> MLKCSLCYLASKVTAGNAKNQAGHPRRKAKLFHVVPGTPVTPFEKLKEQRRRFGQDRHSRLPEYRPGNNVRMDPNTYTLYATKKGVMTIRESRINPKYKWLDVEPDIQKVYRSRELRRALQEREMASMAVGENSNYRVELDLLLEPDWRERVMHVPKATERFKDPNLFTRGVVNELSPLDRYSYT;> MLRNTDVRLFSTFALNPETSVAPHGPPRGLVNRYVSMGLPPWAAWCNKVNRYSLYRMSGVTQRSFLPKPPQEMDVIWLNERVRERVRTSRQVQNVYRQLKYPYVKTGIHYSDVLDHWVQVPMVEAAMFEVEKDGGFDNFILKRSGPELRSTYGERIRRHILVRQKEIQKNFVLQKQAQMLVESMEKEILPMEDGKKVEEVLEKYGIDKEQLLRDIARAAVAKKQQLASAVPQPSHVEVSTN;> MQRNLTKLSAAAFYEFVDNNFLNNKRPPVPGGSWTVEVLRNKSLADLQHIWFLLLKERNMLKSMKEHYLRHQEELGAMPAPSRLKMIDESMRNIKRVVKERDEEATARAVEIFKERLKRGIYRYPPGPPPPPGAHDKTSVVKVELSCYVEEERLRELFGRYDVFEPHKGIVRVELKLPDEVLKQKEEAEQLWTQYMAECSDVKAYHQWSTAAPSAYDYTEVELAPGIFANDAISDKGGKHSGDTETHEGVIVAARVPVPPPKEKQPPPKNPLERLKAERRSYLARTTIQLGYFPNVTLPPPRYETVEAVPRPVHPDEIEGPWEAYITYDREDGLSYAQSLGITTIGVATVLGLTEHVREPQPYAVVDPVYCEALRRERAREETLMKWPHVPEWKYEYSTYTRKHLADIVQYNYTNVVDYVDREVLLTGKSVWECPIHIDHTCGGSKTVPPHAKKPVRYMDAGIANVGVTDI;> MMRRMWVPTFSAQQQHLHHAMVLKMSTYASTPSGNGVTSAASNEEMNLHDAAAIAPGPYRRVGNIFIVHCDDHPFKHSWEVNRMLRELRLEFKGQTTIVPDIPQVRKRIWRVRHIVKVDVLDLDEAKALIGVPEHISFTDLASQLPPSFGRVKAVPSPVIRSKMNFMKLRRMRLRDVLHRDALELRLLELKRSAMKNAEQQKHAQKDERTDNKEGEKC;> MVLHKWAVVSRSAPPPRGLRPIARTIPTHPRLRPVDYKIPYVLRTFIKDRHTSEVQHLENRGMFAEELSIERSRFPRFHSTFTIQTDGSLNEREFEFAVPPIVTLFHDRLSAHRERQLELAKIGKLRKERNWETEQKGEESVSMACNALAFPYCIPKNMLKRSRVVDPLNSKSSTQGVTSGGG;> MFRRTFFTPMIAQPTLLMLGNKGGTPKRKKNPMQLRRKVYGLHFKEKYLKMEEWYYCPLCAEPKKPGEWCRREDCRQIKP;> MLSSTALLLRGQYKTRLKKRMVGFIPKVIPRKIKNNMVALRSEANTGHMEGYLKTETERLDATGRKVQKVLWDPVLQRHCLFKETKIKGPFMTKSAIAKKVDFPIGGAEKMLKK;> MGSEESNNICAYKRTISLAKIYIVLLVKTAMLRYSRLCFPKMGCEEITRKARRVQLQPTEYLAQHRMQVWQLRFKEMGPPFSRVWVALGGKMRRRRVGRQVDVKDMRYYWRPIEPQYQRLYMSRLRIRDHSNKLRQPMRLRATNADIGSGSSSIEWERASNRKYGAMLAPPKRQDFEFRVV;> MRGTTKPMLFLCSTAVRLNFFPLGLSAGPLNSHILLPRNNFDGRTTHGMKKIQGQSKDPQMVMSRDELKLRCEYCRFEWIHDTLCVRCPAQPSHDQREMWLHSTWMWGKQQPYKYYKYMPAVRNPRTGMPMAREDARSMNNERRGQGLTTRTLNLEKERRGISRDVSRIGQYNTRWKTRFPFPT;> AAAAAAAAAAAAAAAAAAAAAAAAAAAAAAAAAAAAAAAAAAAAAAAAAAAAAAAA;>AAAAAAAAAAAAAAAAAAAAAAAAAAAA[2x];> MRSLIAMRRRFVSGTWTIAVSTQQRHRSGSGPGDKRIRTDWYRCYPSLMREKDRDMYHCYYPYLFDHGDKMSLYPKIPENPREWQPEQLQTTYDAIREDKYDAFIRLREKFPELYQDTRAWDNPPPFGEFNMFYSVRFGMVGVKAFTCKDYDELGNQFDCTAFWFPDNQVVKHSTRNGEVGTDKVYVGAMNVPVEFHKPHVAAFYKAAGVPVKHVCAGFPITPDAYAPVGTKLDVRHFKPGQEVTITFQNTDYGFRGVMFRHGFDGGYVWLGDSRWQRRPGAMGTEGQKRIYPGHRMAGQTGAAAETYQGVPVWRIDYKNSLIYLPTLLDADVGTYVRFSDTINTKGLTLWNEHRGLPAFPTFIPPEDEDLSKLATDECQLKSPPLYMYFRDEFPATQLVSQADVEDAKSAKPATAPPKKKVYDMKKYYEARKKYRQSMQKARKYKLMGLRTKAHEKQEEARRAKILKYKRMK;> MRRVSFSVVLATFGKRHSSIFSPRYDWRTSGVHDIAPRDEGDFLYQGPQHVLPGAHPLPLHHPHNTITRPVISPYIPSPQRSHPYFTAPLPELPHFSTTKPIVYTYGTMKERIIAPVFNLKNEVIYTRELDPFIFGMYPEVEELSKNLTYWMVRCQNFASKWDYETREIWRKAKKNWPNTGMGMPRVGNRKNHLYTWGGRTKPSKPWNMLMPTMDVKTWSKSNRMMLTLKMLQGRLQVVDRLTLEEPTQECYLELCRNMSWDVRHTGGGVLFMDGGSRITPSSEFDRAFFFGSFFNGRNKIVRPTVLCDEQYDYNKTAAKQRMKGPKGAKNPIPINRFNAYDAMKHDRLVITEGALMQLEDELYEHKLQILPPHIRNQLPEYGYLDSEALGDCVPSLKTIQMEAAARTEEAESDMYKSFIDNPYNPWKDNMDASYAVDGADGTVQKFVDGKKVSWSMLS;> AAAAAAAAAAAAAAAAAAAAAAAAAAA;> MRRTVVQRVAPWVPPPRHDIKVTMPPPPGGEVGGRFGVSQGYSDRLARTPYWKRMALSTYKLRMMENATRYPMSEHRPGEYDIRYLPTPYPCTIRNRPLLEVGEPRQIPSIRIPVIFLVNLFDEAKGCWFGRRYETVYVERQFMREELMPQRYAIYATPEAYKLLGLPVVNHHTHEEIPKTPREYEKLLERQRYDEERWKYTIEYLFRKYEDGPPELLDRPEDGWDGSEEIALSSVAGAGRDGVVSQRKGPVKQRKARKIKLF;> MSPASPLPVAALSRLRITHRSFLTRSRGRHVCRSAVGVEYRPEQQKKVLDHSYARVINAEVVHGDEQKFWGERRTFYTQRNIFFPMWDRCAQALILITREVPRVPQEMAFRLMAVFLKLMLLPRLMMNTELMLPMWIASNAEGAMAAAKDGSKGKEQSSKQQGESKDDAKKEGDNTK;> MLRACGVLQLRARPKTVCVEPGSNRLPEALVVEKARDIFGRPEFPGKRVLHNWRFFIKAGKAATGPPVGQEFSKLGLKAMDFAKVFNDRTKPHFKEDVELIVRIQVYFDKSYLFTIEPPPTAWFILRALRKKRRETGPVPLRGHYCALMTLEMAYEIAKMKPLCWGRPEYPLLETRVRRVVGQARRMGVCFIGVDTPYSSPVKDMTEQQYTEECERYRRIHMEQYTTLRQRELEEAPLIERLHRPNMSPLTDEQIEEGLRDPCLLDTLWRASHPLSPYHRDLRERELARRYLNARGWVKDMTPEEMRIVFMNYRLPEGEKRKQMDEAAMSGEVYWTRDGAQL;> MQRSTRIVMAPFKSVLRRHKHHPEGLPLYNDMSKQWLCREGERWWLLDARGEQLPRVAAVAAQYITGQHRPDFTPGMITGDHVVIVNIKDVVMVGDQWIRVPITWQTAYPGGKYRIRLTDMYERDPCMLMWWFLKDEVNRHFVRKLKTRIAPLEKAWLYEDSIHPHADKNPRPLCWTDPEVKGWKYRDPQFIRRWKPNEFMH;> MLSVSPPLRRYRLFHPRREAIPMHMCPAKTIFPLINSNNLLVKTRNSWEDFTGRKEFDEDHPLPVVGSRLNGRTTQHKWNHWDQYLNPQITQSIKDLTPTPEYVGMRCGHNMIKMGWMKIGGSWKYSRGYNDRRRVFARGQWQERKMTPRFMLAPRVSAGGPRNRYEGKLVFSPLRLSKLLWAIDTGRINPNEVITLYHLRQANVVGEREIVWPGFVLISNGVRRVPYPIHIELQNASAESIRLIEEAGGSFTCVYMTHEGLYQELHPEEYPIFMDQELPERRGLESLATNPSKRGWLTRWYEDSSKYAHPAAGRRYSHYLKPPTERDFPATVEEYEMVKHHQKWHLNQPGTGTLLPWHSYNTADLVKRAAGRL;> MPSPFQQTLLARAYHYVHPKTGRPIRQFRRYGDPRYINNEAALIRGQWGLITADFGMVTQSQMENARLAILRRLPRGSFTLTMHTDYEEFPVVKKSPESRMGAGKANIHHFAFKFTTGVPLFEIMPISARRLNQAEAEGIFLAGRPFIPLQTVVVPQGRVDEYHVFK;> MLRITLLVVGRAPPVIGCTRKARYAGIDDNPTITYKPWDTTEPLMADYGWTRGKLPKFRARSPFHRQQIARRMVTEMIRKDYCIVGGARAPALRILADHVVELAKAGDTDSRQQLAYFLHDPLMVDKAFDEYPRRFKDMNAKYAMMTRLKSRRRTDAVAMYFVEYKNRDMSDNHKGEDYSAGPERFFLPPRIVETEKGIQRPPHMQMAFDRWASKFKTEEFHHWWRLRHAKLRYWGVRNVPHPSDVDPLWTEKEEEEWHNEMLANTGEYEDLDLDDESYTAAGEGGEPSPAGDGPQPQRVG;> MGYTRERTNRHFFVARANAFFSRLPIARVQRSLAMEAVREGRMRPWKYTKEQILGAPVTCNFEYNPRPVRLIGTVMDAHTEETSIKGGLKVYARNEETNMMLWIPPGNPKLRHEVTSTKGSFQHYLDERDKWDEAWITGRARMK;> MLRRTVCVQHYRAKLELDRIRSMLRGRARLERKVGLKRLFFLMRTQTRYRVEQQAHWERAIVRKNVDSAAREHGTGWQHLRNELGRQNVMLLPRSQQLLAQYEPLAFRAVVELCASRIPPPPPPVVASVPEESYTLWPPASHDNSECASTDGSDAPHGQQQSLSHPAARVELRCGVERVLRRGPSGLGNNVNELIDAWKEFDVSPLRKGEVNK;> MPSLANGLRCPDALITRTLNPLLNGPKFAVIYCGNHQYKVAVGDVIAVQRLRVEIGSHIALKKVLMVGGPRFTAIGRPLLEGVRVTAQVEEQKRMRNVVSLFATPGRRHVRWVDAPHAATIIRICEIFYSPNVVGELDKYKGELLETFTPGQHTNPVYPVDDGYDVFRKKDKEAMENATTFLDLLGGV;> MPRPAPRFAMGHMLPHRSNVGSQFLHTQRHGSRSTWYKKHYFSLRPFAIQRHHGTTPRILLDRSLWKSLWITKLQLPDINRWERVVNSRRVTEDRYAFVEEEGVMHKVNWGLYCERLETELTVTQERLPQHTLLMKAVPSSWKKLDIDISVIRGLSLREAMAQCKLSLRKGHQIVFRALEMAQQGAEAKGLDKEHLRVAHISCYPGPTDKQIDIRSKGYYAWKTKKSSHLVLTLAEDPEMVLPDRTCLPYSSLMSMKRAGLSAQPTVIDVPAITADGI;> MVVSLRRFHSYANSSRGGATTCLITGGGKGHFALTVSTRGRFYRPLVDDGINLWRRRMGRIHKGWRTWEYQHTRPDPRPFPDPPVNDYFGRSRIWNPIACKLGYVRKKADEWGWPNKPPPPTGLRHSQEFFPFFFERYFPDAEVRLLLDSVLNNETKRPVFQIPCSMSKVELVNYLKNIYGIDNVVRVEVRNRRGRRYKNEVGEIKMMDDYKVAVVELDTPVSVELKQIKGTEDTSDNRPQERITQ;> MYARFRTRSKFYFRPARPALAYNVDPNVMRRPKVKRGLLKGTYSDETVDLRDRERLELLESMRHPRERDFYQDHTYHNQWLRRDLEKHQKQQLAARYKYFAPDFEISPWIWYPGDIVEVVSGEGIGQRGTIIAVIKYKNEIVVQNINVQDVVIPASESRPEQIVQREHPISVTRVRHVDPSTNEICNIEMVKVRNKETGEMEEKRMSLESGILMSIPPVNDELEVGDPLKDTPIQDADEATYDREAEQAVLVDKRLEAMEEHFVQSLKQSYEFHEPLRRKNAEDMRQFQTDVIDMACAMLGERLLDTVNASDTSSFPAEWQEAIAMHVEEIEAEMEEVAAKEMAEAKEGGAAENEQHDDDLDDDEDELDTSEESVKHV;> MVMRRCSYNVHPTWYMMPLRAYHMPGWKTKVSTKDVRTREQREADRKVRQIEKLPRPQALHDFQYPYEKTVLSDTMFQYPVYENELDTPHLFNITEPPDFFVYWNVSDFERTSYPPLPEEDHRLLLPLSGSAPWKQHRKRSLKYLRKHEILPNYLPHVRQDVNLSVVFPGVYATRARLCEETGEPLPPPPPVSRMTHRNFWMTAHCGNYIELADLQHPPSIFFLDTVSATGQGKAVEKDATEEGSDEVWYTLIIASPDYPFRVPASVDASTQRGFFLNYMMSNLKGGGNSTVLEEYESEQRQNNQKRQHLEELVRNPAPIAKEGDVIVSYTPPLPTEDAGTTRHICMLFKQRSYVSGASCALDDSKASFAARANFRLHAQHRDGIPSSSVEMLSRIEQVLPPDPSAVTFFQTKWDIQVQEFYESRGMLEPAAPLDEEIEAILAYHARKPSELRVRARHRPDGSTNVGDDPNFWAQAEPTRMMDGSMLSLWSRRTTLGANGVPITYRR;> MVLPRKLVGQCCLLLQKKQTAASYMANAGKVGNEEKWAQAAMEYLHEKRHCNDSRKRQHDVDNERRMAFAFDRYCSVNEKIFTERLSRLSDRMTEALETIKQLGMDHALEEALMLSSEQPPLNFRRPTLTPPVAGYEPGFGLDVPQLRSRQAEYPPVGRPTDAMEFGEEKDPSFPLVESFRVEDLTTQCLNELEERHGEIREAAPTTGVEGEAWEAYVALQKKALARQQLIFELCNNGELRERYDSDVAFRQRVWEERGMLPLEIERERLHEEPRHYAQEPAYHPFRKM;> MLRCSCACRRGVYHNAPSVYPFVKPFHDTPYDQDRGRHDSVGQRYRKNSWPEWMDNGADGTGYGIGLHRTHPLSRLRGNLKRSPSHVPRVLGMMIQGVWHKSGVKLYFRGGKPPNPSVHPYLTGEPCPLYGWKVTDESVIRQFNMPSIDGTNFRYKPYVALQERKIMGVQVPSDSVSLASGRTTESKPLAKRLFFWR;> MLRLCRVSLRVQSHQKKRAQHPNAGTRFGRVYNRGFIRYGFGGFGMSVYTPKKDRRFRVQPLPSLHANSLADDTPLVTTTRTLSPNFRAFALQDGGVFFTHPSHEQVMRVGQNILAEETKATGMTSMDTYVNSRIQSIIAENTVENVALSHWRRRHMWNLVRTHGKLQRHWGVSDATKGARSNIYGRPS;> MSRNGELCLKKVIISYCPSNGAPNTRQFLATHLPHFHAKYPSVSIDLRPRLWPEMAITGVYRDGSERSYNTKNLSPMGIFLRLNNLVSTANDYDQPFCASHLHFQRRSVQGTWNPWLWNYETERRRTEAPQWRRKLSEKEWDYYVGQYSAQMKQEEDEIQRRVADRTCVQEQSTREVQERWKRHVVPRMQTDLEFNLSHFKRQHARGQLQQRPVTMGEYRLFSVPDPRELGQDAVDTMRRRESHNMEVWWRKRKEQLKPP;> MRPVARLPLSRVLSGCRGFHSQHRTPVLPQVPAAEVQQAASESKVRVAYLLHRQPVVKPTPHPLEMEMAFLLQREHQRYSRHESSESATHFMAQRGQSIDALNRTDPRQIQSNFFGLELYQDAMRVVLQRYKPERRVTPRDLWDPATYGSSNANSNASSPPTRHSLHRKLDDYLHLIVRDEASGKWTVPQTELRGRETLRMAAERAIATDNGEGLDCYVWSNAPQATVPNANDGSWLFIYVATYLSGRPKFSEFRPKTIDHAWVTRHEMMQYEENFQSPELVRVLLDISADSTFES;> MLNRSRLRRVWLGGTAANTSLGRDVMPSTGKYINIVSPTDVAANISAGAMPPEANVAAALPVPRIQYSKWNRALRSDVYDELLKLPLRYKLHDFAKLCPPQRCQEEPEAVGVVGRDSAVGYLPPLGPADPLDTIPFFVHRSSNGVLPGKVFSMHPRNLMPAFYLRIQQVEGDMFRFEEELLKIFPTKKIFVRSHSIYVYNVALDGRMVLHHWLLGLGF;> MRLHTVRAPIITRAAMRGYSEARSNYDGTSLPAWPAPGKKPTYPAALSELRLPQPRMRKTRTEWMYYHGHGGCPGKYGPSREIADFEYADGTPASISGRRFAFKHHQDHLLVQLIRAAATVERYDASGLLPRIPGTAEQRNWDPAIPLFLDDVDEQGRPAPLRTAGDAPGTMVSHVCSRVVDERMGTPTHTPNELANRHEGETLEANTMFATNDPSAFVSDTVKLRDDKRPYWSRRRWALTDKFLVPKSPKPKNTIKDE;> MLNPPKHYSVESLRTVGLLPAQLALSRKPRLRPHVGNLKGLVYPLPYYAMWRGNHNKYTYNKSTVCLWGEGDTRSMYHQHYAHAKCPTDYGRGGREFEYLTVKRGKMLQKPLPRVQYVAEGSKPVWLFKSWHTPLSSPSMWEREVQYAEHTPEHIGAKRPLAVVAPRTMHRYLFLMHMEKVTITVSPLLFGYGHTIQKAVLDFYRRAISARSPFPKDKVFLFYAIDHITPRIEVTWLDGTSYVPPVLEGASSQDLIQMVMEEAWLAADRMAAEGRVLNPLAIDDYKWDQLVVFKKVRDKEASKGGGRKK;> MLRHCTAHRRYRTAWRELLHPLPVRARKMEWLKRDAVEENEEILRRPYYTIKSYALPPAVGRQESIHNSNNIRGGMHSSHSLDLIMRQPRRVKTPEQLRALRDRLRFIGVTGPMPQATSVSTKSYTDTYGSRLRPRYPESWDTVPPHQPSRELL;> MLRGTRGFLAVSPGVGIAPETTPVKYTPMMLNIQNMMWWNGKRNLYRATYREKTWYEISRTGAFTKGRRPVMRQKYSREALQAALAMVPPGFEVADVPRPPQRILAQSEGIVGRWYSNYWTLHSMRYQCLLAGVEWPLGERQRPRTNYDEPFFFADFEESKAIRDYRSRWINVNRSLVGMTKRMKEAEEEARYMQFRKLQDTFWSNRKVLVNRVKSMYNQGARTSAKDMPIKTINIKAFLSE;> MLRRFALTSSVALRLRFERDSGHNTVRYRPIPESMQPKHLEDNFTPFPLPKFDESLEYGPVRLRNIPDIEAAKERRRGSRLAATEVLLQETLQEENQFATSGKGDGNMAIAITERHTEDVTTPAADSRFPSQTMSPCSHEEEMRGYVVSRDYPLIDRLHCTRSIEELVAQFEDRPQIESRVAALADMASTVSFRSDEELLRMFTAISAPFSVDGRGLNFLTVKVSKFGRPYYVPNSLLPAYVNLVDATTIALVREQPWRLSASPALFIQVLQFMALIKVFEPNKWFTFSDHAPSNRADYRHAIGVNHSTAFWGTGEELYDFMVELLRVEDDGRIPTMLDLCTREQMVDLLSGFCGVMPCGKAVGDVFKTITDAFLRRVRNDISGPWSAHDWAIVERMYLVTVLCDAGNNEILQLLLSDTASPRGPDFFAAVSRTKDTPTKKRALCLLQEAIDNASAKADKVTLLGLLESGSEFLLSLVDKGVAHTFATQNLFDYRILNSFLHCSLVADRLRVEQSVITSLIPSSLRDVQVQMLMSNERNALNPLTSSLPGNSGAIATAPKLKRPLMTMLSQLEYLNSIDSVFILHSSLMATSTDQLVSAVRRLPSGKDSLIVTMSCLRALSVKSLTSPSMKERIACARALEIVSYELEKGRAVLLPFSEEILLHDAGAYCDEDLMLWTVAAFLARELPLVKVHTLMHSNCTARTPYRFLKGGHNLLVSSRSLYDKGAPLLSSLHSKELRLVTHNVRLRTPVRDRKCTLQYYNPIRARFVYRRDKPLFDKYHVTARNLAPGFSRGALKHDWRALGVYTPDHPQVPYHPLQTWMLGETTVEAE;> MLYTRRLMTTGGSATADGAVSYSKGSYHIVPKKYTVGKRIAVRSYLDRNRTELSDRTYMPQKAWFEPYTPKKFDMEHQRISHNFYNLETKLIWTAFDTPELIGILLHDETIKGAPHLYDAEFLESAVHWTRESRYWRCIGITKPFYNKTTLRAQCWHDRGLQVGTLVFSQAMRDALMDLERAVRRKELGLEPNYVWDRWGPVGFIDGARTDHLPRFAHNPYVDPDGVEVTEVDIAPFNTHEQIKERYGAFIDPDLRPFEGVFRAPSHGALTLDDVPHQEAVRLYRDLMEKADMPVMLGNGAEIPPMDMRALFHLSANPERMKAASELSSWREVRGMLAPVQEVCDEKVEALRLMENTRHDAARVRTFYEEKCGFSDFMRTPDKVITAAVLCYLQELQRICTETDWGKPLARCLTDLERVNVMGKDAFLVYRHIEDAILDKKRRVWATRFAGEANEESTLDYLLENFGRRTEQTRNVGTTGTEFDREQEPIGRQVQRRVLDSDKASKLAEVRQKRGKMWSNKKSVFDSLHQKQLQNVTYGVH;> MLRRLAGCVAFRKNVVRPFMNSTALLSSPPAAVSAPVIPKSGNEGKDYSVASGSVDTPVLDQLVGYYVNIQSRKMYYKDFLRIEHQAVRWAFADIRKNSEALAHGLLQTGLRPGQRVLAIQPCNCETFVLQLACAKIGALLAVVPHHNISADKLRFYLNEFQPHHLIAREWIVVPEVKQGVLVERNMHFWDMIYNVIPELGLSYPGQRFQWVHSQEFFFLKKVVITDHNMNLLGVTPMRKMLVWGPFSYYEQRLRRLSALLHPDDPILALEDPHPALEDKLHITYSHRNCINAGFLFGNLMGLKAESRFGVMPNHHVDPVGAIVAPYAALTTGAVLVHIHSDMFTDDHAINGIEKLCVEEVVGMLGKKSDFDLLLRHAGNFDADQYEHLKWVVLFEDASEPTVGDEYLQKLAKELGLEDVFVFRGPLESAYMVMWRSLKRARWEMVPHVEAKVVGDRGTADARILAANTRGNLKLKGPHISAGYYNNAGLLTELVDERGFCSTSREAVMDERGQLTLHGTQLY;> MCLKRKAPHLFCFCLWSIFLSFRCFCFRSYAIMLPLLSFPTIQISIFLSFKLPITTFLLSPCFVFVFVFAIRYCGELTLNAQLVLFLLYHCAQTQRGPLKEGEMPICPGLCGELAAVPFRVFLGTLPTLAVEERFLRQLQPVFAWYSSRKRVKEQANEFIEIDLASCDAELLLRYSHIYYVRRQLFDELIERQMTLLDSGKAPKMAEPSLLQCLAGCNMTIADRLQLEIRQLGAAKRAASVPGRRELDPVARLEVYDYACMMRLVEEDAGAVGDAEMKARAYLPREVIESKLGHLTQLLLGSDARAALDKKDVKLLNRMIPPDYTRVGCVEKLRPFDVTAYFRFYGERINNVKVENYFKRALWGHVYRRFATTPSFLSGVSTYWARHSGLDASFTTTTMPQEVAVAVCDQQIQFPAIKFRAQYVYTSPETARQLWRTDAAVPLMRLFPLMGSRTAEDLAAGVLTDAFWMHLGLSEEENLLQDSLLLKVRRFVDEVGDMYETNIDSVLKRVDDNFKQVVPQLKAEDLQVDAPLQDGEGEDTVRETVAA;> MLFRSVSCKNYQRGGWSPGSKHQKHMTLNPTLYLYRFPGPHGPGPYTMKYWWTLGCFPTGMEVPFRLHEFLSTYQQEHVPVEVEEWLRCYIKDPLSELVNASNDFFKAVEVYPEVESARGYKTLQPSIAPLLVPMKKFEEQLGVKISPVGLRSVLSNPVLKDRFLDDLFDYKSYVEKGGSTPHRRLARSRFEGSLSVLGECEKCLPEQHQVEISESLGTFIGATVSPAETTADDERSLILLLTTISEGCINAGNYSDAASVLADALMFCHDPDSQATTHANISFASLLNADFKGAEYNGREAALLQPQVKPTSTACARGYVGWAAAAAYQDDFEKAEAIVKDGLTLYVGNEHLEKLANKLQALREEQPSVYKQVPRSLRESRSHLPSQQSRGLLSGSGKGFSNEFDWVEFKNKLYPSKMDPRNNEMGSVFRRVGDLGSFISTSRSMERL;> MSRSAFSSRGALLFSSAPLQCQRRWVTRLYTSYYTGVLYPNQLVQPKQRLPADVSVSAILQKRSEPEAAAERGSNKGDKVDVSKGEKTPRVSWDDADSTDVMRVDNTQQLKEAPQVERPYVPLGEVAKLELQGDYYMEGGMFQEALEHYGVVAKAYNYAYPENHAQRIGIRIKLSAAFRQTGRLESSLANIEEVLRMLDASTRPSLELICEALLELGITREALGMKREATEAYEEALEVVNSFHNWGESHRMLRLLPRLGRRFNYNFEEKFVYFSPFDYDRTFALVDQCLERAETIFNEIGDVEGAIRVLQQRKEMIDKKFFNMRDFAGRIHTMRGHWKRRAQHLTNAPTPDELLRYSPTIHQVHRDFKYELTAPIGREKEVMPGVNRLVLDMGNPYRRRGRLSNKMLKDADHKFANYVRQKEYNE;> MRLARTLHHVASATTGGGQMLEGLVNDGPEVAHKQHASFTPFSIQPWQARCVGASRRKLLPQMLMYHGARLGPRPLIILDHSTKGEAGVAEAARKYESILSQLSWDYGAVYIPLHAQCTDSSKDLLEQSCQRICAVMDALDVRWTHFLTYSYGALVAVRMASSQEFPHRVGTLMSLDTPLVTREFLRNMEQREDIAKAERDINVPEDGLAFAKQALLSSLEGPLPCPAAEDESLYRDYLFDPNRIFGAGGLVRDESRYVPLKSLLGVRHPVQLIVPSANPLSDAAAHSEVFGHRRPAVVKCCQRHEDLFKESAAKEVAGVLGAWMRRFEPDCFISKRYEQAANEMGQLMLSTAQVSSESAGKGGGEPRKKKEKKKSKA;> MLVPGLSLTRRAVTSSCCRPLHVVRGFSTTCTLFGLEQLQDVPTSTSRRPTGLHRGPGKRQTSEREAAQYKFIRRWELQMRDEWDQLEPFKGLPKPKRQFGNEAAEVIWPYALLLERVVKVHPFTKSIYVYYAQRQSTARGKLAAEIARSFAREFLIPITFHNSQVYTEAEMLLEYSETPWVVLHSLDNGQKPRILPVAPVEGTPAHTAVEQLLAEVVQGCEALGASVADPVTATRVLNERPLQNQYVRVDYQWFGDTPDERASHLVRWEFEPEQIEPKIRHRTRHVLDWLNYDGNLPTHRAVHVNAMREKARQKAPRTVAGPRTFYNSAGSRANARSSRFGGQAAVGK;> MLRRSDLLLKKGWTHNPGRTRRGGKNLAWRPKMSERTLEQFVPLHLAFPRRHPNSWQERQFHLLGYVKWPKEIGFYNAGDNFELTPQAAYRIYKQNCDETFWTRLHNEKTIIHLLPLVEQDPGTNMVLVDDIFRHHLKRFGADHYIYNAVMQAAAFAKDFPRCEQLLAEMRGLGLEPNAQSYVNMMLGARLTGKPRDQAEAFFREGIKTGAISAVMRLDTEFQMWMNQLERLGSFKAKVGYLSVNEEGASPMPRDMWALWGWHRTEAKFISRKQMISEQVQNRVRSGKELVGTVYQKARRQPWAKYNGMFPYDYNGPARRPAASFVDAPTPTHNAEVCGTAYA;> MLRLSSWNLKSQHHNVLRRSRPHIHKYRELNRWQRQAQGISKWDQSHSHRPLPYVERFNPESVGLTRGTSAFAWKWWHTQYPWLPNVPPEAAQIDEAQKQERRSHRPPAWDDEFAKVVLNMNDAEIREYLMSKLTDVIFLETQRDGYELRRLDFEGKPLTSLPEPRIIENFVLEEETIRERVIYQVVEGVFRLSPTSADRRELRSVANIIDYVLTHVRAARPTDRERRQERPITSAALAVMQKCPIQPQLGFVHALPHDTRDALLQEWERMHHLDWQFGKAVYTPRSKENVRGNLTWLREDRHYDQRMKFMQEVESGEARAKHMKLIAEAAGN;> MYVFRFHISSFHSFLVNFLQPSRGVGEPSRLLHHLETHPSYMRRVTSTAVHRTVSSVLSPALLPSFNGTLLLSVCFASCSAAPVRNLYKRLGLDHKATSEEVKAAYRQRALECHPDVVDDNQKAQAEVDFRAVSEAYDVLIDPQKRKEHDKALGLERTVPPAKKQQEGEGVGCDSKGSFNRGVTRPRNRKPFVRGDADRNFREAFHGMSLDQVLFRERLRQRRMQKQMEEKAKEGDDGSPAGREESIRRVAAAAAERFAEKVRRQYGPGMLRHARVYTSLSRDPQPPPSDYMPFRPFHGWTVPNGVRTPPEPTLGPTAKVEDVKDVQLAEPAVGDASHQRKLPKHFPVVQASDGSSLLREETIACMERERRLPHNMGKLYSYHRPY;> MGASAGLIRRGGGVFPDAVSLTLTPSRRVYGGSGRGDLLYENPDARRHSGRALGVLNGVRHSSQATMPESGQLYYRKLILHSRPPNGSCAGLQRHCHDTCNWSYLIPSLHRCAESAISAKLWEKMCQLGLEDRSKAWVNLTQYERQRVRDGQNLYRYEVHQRLPLLEESIGWAQLDDLLGWFRSARRAWVRLPTSVTLSRESSEAGVASVVSPSSAMSCRLEGHADSRDTTPGRNQVFDTPERVEQLTEATVHRIREELQRLNRSERSDCEGSAAMRASARRLARDEELSRCVEEELGWHGVALQHRIPVPK;> MRPTFPALGSRAKGYENRVMVYAHRRHRAWYLPPKLAHARSPLANKSPDEYGNTWDPRTGVEWYHRLRRRGAYRHWPWARWNDDPVRQHQELSCRRTFSAAVTGANEGVPLWNYYAEVGQEYGLPSHFPLSFMAPFIHQYTSRAWSRKEIERHLKVVEERTGLRTIQQACDATSELLEWGEEEMGVVPHGLLQHVVMLAEDIVLQNKKKAYRKAAHERGILRTTTMERYYALPHLRTGPPMPTTLEQPSGEFPWGKFSTMVGGTRIHPLYRPDGFFKDNMYPA;> MCCLYTSDVFFWSSLVVSPLPRIVRCVSAPQIRSIPCGSGDFSVMKRSLIARWQSGVHTPHGVVYRGAKMKNWPEQRIPENFKFTEEQRFRTKAIPRDVGTIPRNFVLGVLYRHQPCEVGGLWEHCTNDPEIVLDSKRHLREVLKQAREEGFVTFERDAISNEWLCFLTRERYEEVQRIVTAKSEAVDTHSGLRGAAATETSTYAEKFREMNVEAKEAHARRLEEEVANTTRYLRRFQQREIDYLPYTDLNGKVNFMWWYETRDVQQRADEVLTDSSSSKALAGEEEHKAGSQLEATTASTS;> MKRLFPSAGVSVVLTSSSIVMSCPCNHIFTSRRAYYWPYNEDFVPEGAETSRFQSSGSPGTRRRVLQEYALSPLFGARVPCCVVGTLRTAKEIIVLKRDIQSLLCELMELPQGSVTLGPLQQLREMMLYRHGTPLSPRLGDERQLNMDAYARRPIAARTMMDVFLAEDMSLDEIVNFGRLSLGKLQIALNNLRKENAEKSSADCEDGSAVEPAQLLVDRMGISYCEIPSLDESDYVFAEVGGVAVTDEEAERVAQRWAERCE;> MRRCAACLTSLPVSSPTGAAVGAPAAPLKTQAPSNRSLLGYPLRRAAAMEMLYGGICIQHLAQPPFPLRKIQSESLPPPSLQGERDDLELEVKDSTGNVMGYRLFPVNIGIRARTESVRVRSEDCYKRFLAQKHCAAAGVPLQFPAPSSITNSNCLATPRAASHFHPPSSSLSLFTRPADSQGGDVGRTTPADVAAYHPRAWRPYQMLKPMPHNWGPAVRSSGVRGPHMQLLQERIDKKGFGWKRKSRSLWQQDISTAGFRPKRYF;> MLHRTRLAQLINGRILQYFVPYERDEVNPVVFMDVTVEGDALGRVSVELFHDIVPKTTENFRSLCTGERGYSQCPLFYKGIPFHRVIPGFIVQGGDILLKDGRGNVSVFGFPFPDESFEGKAGKHLRGTVAMAHSAPNQNGSQFFFNLARNDHLDGKFVVCGQVIDGWEVVDRVAVLSGSSCGTPVSRAWITECGQSSGDKLEDTERALSGERALHTMPGKEVLDILSPRY;> MLRFTRLFREMAPELQLEYMPVLFTRTILGPQGGFAGEERLVKLEVARKYMEAGHAVTPTEELRRGLWCYNPDTDKYDCFIERNEEFLDFAARKRQWLDVYWRVNTGYLLFGRQSWGQGFLINCPLRKRDVAQKLWEQYKVRIDPRLIEFREKDRRTGIQELGHNWCWLYLPGAEELGINREVYDNKRVKVRIHVRKMNSMFALY;> MRRLGVFCRGQRNSPLLTRGIATGGRVTNEDRRWWLVHLECAPDITPGTFIAWLDCCGTHTCKKLIERNIWTIEQVAALDSDQVDELKYREGCLKMDVVWEHARTIITPLRQREVTGGVESELQGRIMELRKKRELERRREEILKERANVSEQREETLRKLREAIAAKKAAMXQKKQAASEAYGGSSDGGARKEGAEE;> MRRCIPARGGFTMKYKKGTGLWDEDHVNDYKTNRYLSARATMRWYQEMERHQTRNSLNARRATQSHNNNRGLHHTGRGAFERELERRGVQVEKYPLTTTTGTMRVAELVILRRMELEKRAEEALAEQRGELQKKNPTPSEWYDESKGPLNPNFLRSMRSHYEVDIANLPDTPLIRGQREFFIGEERGNGAA;> MLNPTFSLYRKTLQSYPVPPKIRHYDRRWSGSRTNPYNRQYWRVIMNENYSRPSFWVSDFRHRYLMRTGTDYQGQVPSSPQPGLYQGFSDVHKLLANHPKPQRESRHLPVLPMTPRIVFEHANEKRIDTAKRMRRDRRRIEELKTLEFWGWYMKLQRVRGRWCREQGVSSRGVYGPAVDAAELWG;> MLQINAFKLVRATPFLLKRTGKPADTPDYKQVYLPYDAAPTERELERERRRFKQAYHGRMEHRKLVEVKEVPLNVYTYGKEGMSLPIAIFKDQKDPVIGPEWTYPGIYENKIAAQHWYTEELFDKESKEAFESPWQQQILDNQVKRRMAKVMFRMRQVNMKAVDLFQKERGSSRRSGGAGEKGKDGGGKK;> MSGAFGCGSYRSVVAGTQNVPRRMTFYPSAYELIQLHKAHREVIRHFYVRDKIFDNKFPGNALANGLFKFVPNRRENYHMRELMESIRRRSIWMHRIKQQREINAKVVENMEVKYGKKAAASMLCFTTPDSNAYFAPHRYQDVANSWPNYWQHPSVNHVVPKPRWRRHRELGGITRVEDPFAVQASDY;> MLRSRIPCVVVTLVQCRAMHGKPTQSHKVRTQHSRRWWTQSKARHLTAMPHDECKSRPHFPAYNEDVDRPMVVPPDAICFNCDKPIDAGDVNSYVWIPAGNATVPTPQGYFFHFGCFKCNRCKYRLGHNKFYSKDGKAWCIPCALGRDVRVPTRRWHTSYVNTHRTGSRLTGHFFPRHSHQMEFLFDPNS;> MLFTRCLLAVTTINSSTASAAGRLIRIRKKSKWIDRRSKRIPHNGKDVWQFGEQPSCALCHVRFRFKQDYEAHKESELHQNRLRWVETMKWWEEIGEPHHQQHAASEWEWFRQRVLPAKAAAMGLSEEDAARELRRAVMHETPRWYSRIQPPNARSEIKEPRDQRWPSSPKW;> MRISERAFMDIAIGTKAPRRIVFKLFPRKCPSAVKNFIELCSGNVSTDTYESGNRDKLISESALPQLTYKNSTFHRVEKGYLIQGGDIVTGRGTEQLSIYGGTFSAPEEVRASVFDKPGLVGTASSSPNAHGSQFFILTAKEANHLNGTCICFGQVADGLDVVQEIEQVPIDPSGFPSLKVSIVDCGVLE;> MFRVTGLQLKNPVVFKQGQGMFSHQLKRLLQKKSIHRYNWDPLPMYDPRKLVHASRHMDVETWREVPDPHWDERSYLVPDQMFYNIPVPPEYKDAYWWRELQARRVQCPVEWVSHRMYNKGDRQRYDFQDLAFRKKFEFSYEEVVKNAKDMRS;> MAQWVPKTAWKVSNLNKRYGPGYITSGFSSENTLGYTHMVHDSHKLREKLSSRKGIFVIDVRDPGERKLNPVPRSVALHHHDLLSGASCPILPQQKSAAELFVLASNESRGLNSAAALRRWGYDSVVQVDYNTLVEAGYVSRCDYATAGTKDSAEQAVSGED;> MFRPTTAIADSFKEHYHRVHLPRRLALQRYARQQSLRNAAKGNVKAEEVPYKYNRWWVNEEHEFVHQYAFVEDPEVTKAKRETLPPVTRENIWKEPQQTFFLPFAPYVRVVDYPKDPDAKFLKPVNIPRWKDYMQRTKPVIPRTWY;> MNDIYARRLAQATMFHQLMRCHGTLWAATQVTKEQMDYNFIREEFMRVNGRRAMPLLLGAAANENLHQLHLSHLSEHCAWGESARALAVQRQTPLSQRVAALGRMAETIHQVKTASTVQN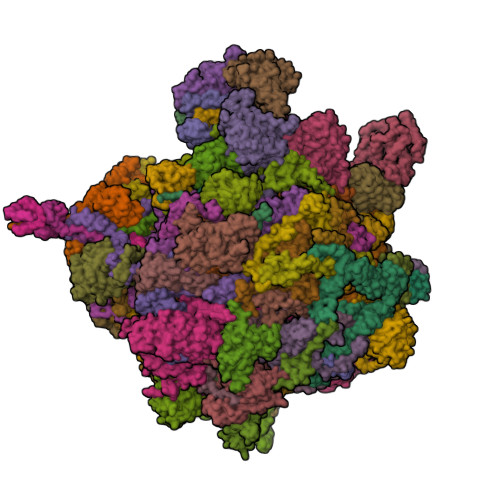LFNEQISCMEGISSFEEEPLIEGE;> MSSRFFQKYFIRCGNCQTIQRYAKGYKPIPNPILFDSDAHCRSYHRERRDCTGLTGTLVTCRCDKCARVHSHWTVMDFQEFLDAKLVMTPEERTALLWPGAGSRAEPSSGTSN;> MVLRGVRLRSVAVSCYGSSLTAATRCLSVRTEDFFSKEAISHARRVSWAPHTTEKKQGAFAKLARSNFGDPLPSSFAQEPYFEEEIEAHRKHHRPDVYIYKYNVSPTHFSLRE;> MYQRTRFLWSSWRDYPLGSRDRRGRFNMDEAAAALQLNPAYAAALYRPLNYTFHIRGQLYPAQKGRPSRPGSLAASQGRMFPLYQRNDRLDKELFRLNSRGLTTE;> MALFSCFRCGYMYEFAVSNSYCRKLTLRNDHCPRCDQLTLFRFMSVSGMVGNMPFKPIGVPGPSYATLWWRKTREGKEASAPLDAVCKSDRW> GAEFKEKPEAPTEQLDVACGQENLPVGAWPPGAAPAP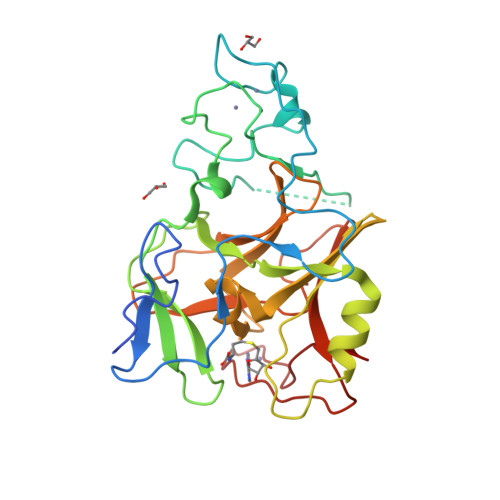FQYTPDHVVGPGADIDPTQITFPGCICVKTPCLPGTCSCLRHGENYDDNSCLRDIGSGGKYAEPVFECNVLCRCSDHCRNRVVQKGLQFHFQVFKTHKKGWGLRTLEFIPKGRFVCEYAGEVLGFSEVQRRIHLQTKSDSNYIIAIREHVYNGQVMETFVDPTYIGNIGRFLNHSCEPNLLMIPVRIDSMVPKLALFAAKDIVPEEELSYDYSGRYLNLTVSASKERLDHGKLRKPCYCGAKSCTAFLPFDSS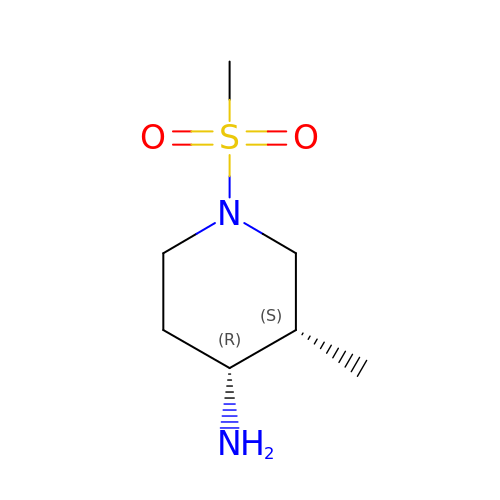(3S,4R)-3-methyl-1-(methylsulfonyl)piperidin-4-amine | C7 H16 N2 O2 S | FRNHPJXWQSBQMR-NKWVEPMBSA-N>[2x]QTKKAAIVELLKQLELGLVPYDDIKQLIRRELARRLQWGYKPTYEE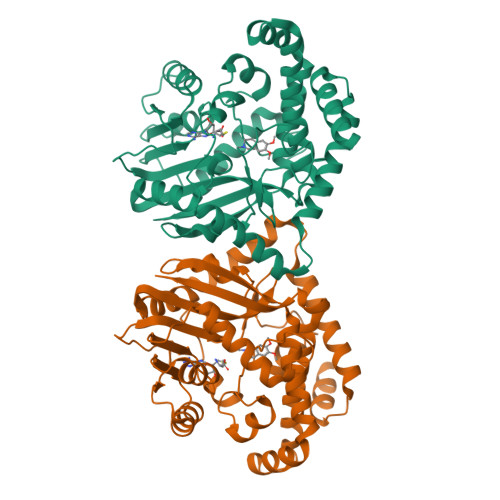QIAEIQNLTHSLRQMKIATEVETLDSQLYEIPIEFLKIMNGSNLKGSCCYFKEDSTTLDEAEIAMLDLYCERAQIQDGQSVLDLGCGQGALTLHVAQKYKNCRVTAVTNSVSQKEYIEEESRRRNLLNVEVKLADITTHEMAETYDRILVIELFEHMKNYELLLRKISEWISKDGLLFLEHICHKTFAYHYEPLDDDDWFTEYVFPAGTMIIPSASFFLYFQDDVSVVNHWTLSGKHFSRTNEEWLKRLDANLDVIKPMFETLMGNEEEAVKLINYWRGFCLSGMEMFGYNNGEEWMASHVLFKK>[2x]GPGSMKNISNKRIIKDLKLLLEEVDANNEANSSGSPHSTAIFSVDTDTIYNWILKVKAPADSVYGGA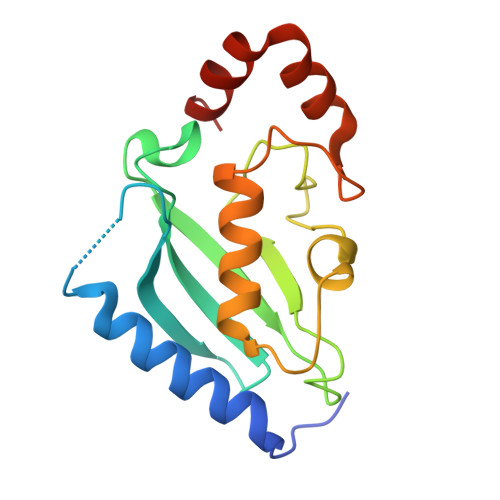GNTYQLSVLFSDDYPHEPPTVRFVTPVYSPLVTGEGGICDRMVNDFWTPDQHASDVIKLVLDRVFSQYKSRRDDDVNPEARHYLEKFPQDFAARVRRGRG> GSHMASMKKKGSVVIVGRINLSGDTAYAQQTRGEEGCQETSQTGRDKNQVEGEVQIVSTATQTFLATSINGVLWTVYHGAGTRTIASPKGPVTQMYTNVDKDLVGWQAPQGSRSLTPCTCGSSDLYLVTRHADVIPVR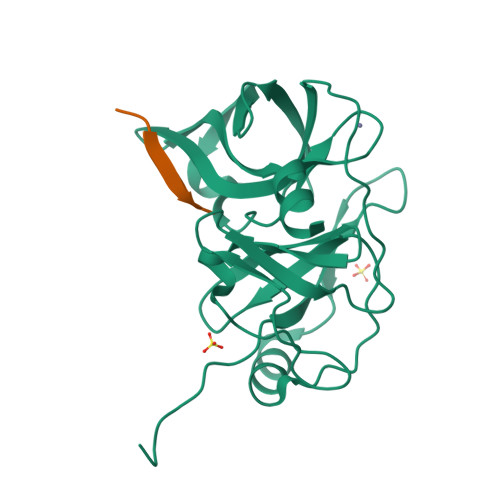RRGDSRGSLLSPRPISYLKGSAGGPLLCPAGHAVGIFRAAVSTRGVAKAVDFIPVESLETTMRSP;> XQEREVPC> SMKLDTRAMRHLTAEDWRVLTAVEMGSKNHEIVPTPLIEKIARLRGGSSGVHKSIATLAKAGLIARMKEAKYDGYRLTYGGLDYLALHTHAARKDVYSVGSRIGVGKESDIMIVADEKGKQKVLKIHRLGRISFRTVKANRDYLRNRSTGSWMYLSRLAAIKEFAFMKALYEEGFPVPEPIAQSRHTIVMSLVDALPMRQVSSVPDPASLYADLIALILRLAKHGLIHGDFNEFNILIREEKDAEDPSSITLTPIIIDFPQMVSMDHPNAEMYFDRDVQCIKRFFERRFHFVST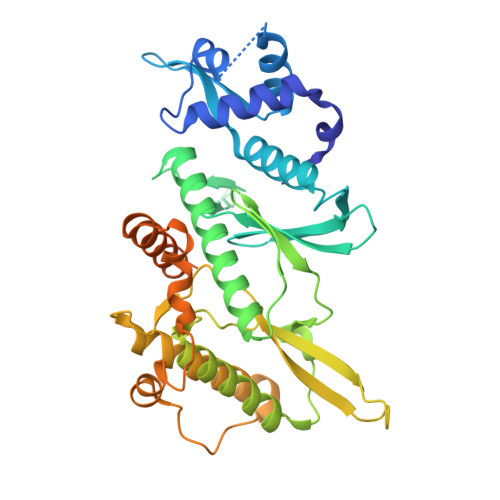TPGPFYKDAKKTVGKDGAKRLDAALEASGFTKKMAKDLEAAIREQQESRNDEEDSDDYEEDSDKEKASNEDTDVDDGRLQVIGDHVQLGTEGDLKKLTINDGT>MAHHHHHHVGTASLPPLEWPLSSQSGSYELRIEVQPKPHHRAHYETEGSRGAVKAPTGGHPVVQLHGYMENKPLGLQIFIGTADERILKPHAFYQVHRITGKTVTTTSYEKIVGNTKVLEIPLEPKNNMRATIDCAGILKLRNADIELRKGETDIGRKNTRVRLVFRVHIPESSGRIVSLQTASNPIEC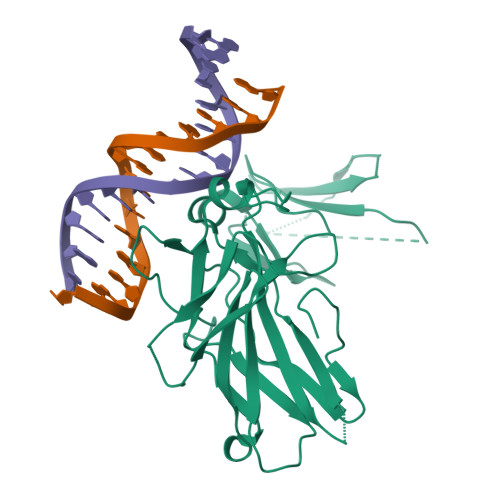SQRSAHELPMVERQDTDSCLVYGGQQMILTGQNFTSESKVVFTEKTTDGQQIWEMEATVDKDKSQPNMLFVEIPEYRNKHIRTPVKVNFYVINGKRKRSQPQHFTYHPV[2x]> MEELTYRLFMVATVGMLAGTVFLLASSREVKPEHRRGVYISALVCGIAWYHYQKMGASWESGSYDTGLRYVDWVLTVPLMFVEVLAVTRKGAAYNEAVRNWGIAATVMIGAGYYGETSAAGSNEYWTGFVIAMATYVWLMRNLQAEGEGLKGDQAVA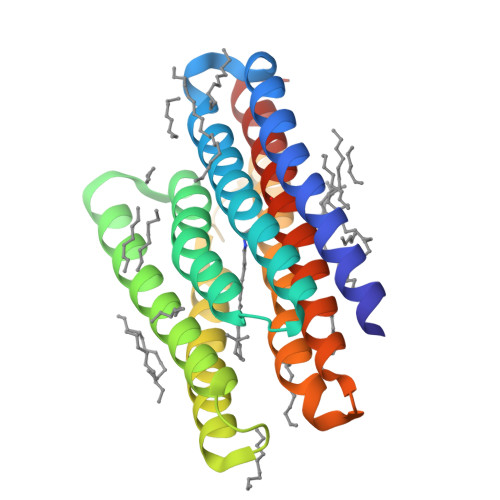FENIKNLILVGWIIYPLGYIAPVVGDFDAIREVLYTIADIINKVGLGVLVLQMARVQSGEKVS>MNRQELITEALKARDMAYAPYSKFQVGAALLTKDGKVYRGCNIENAA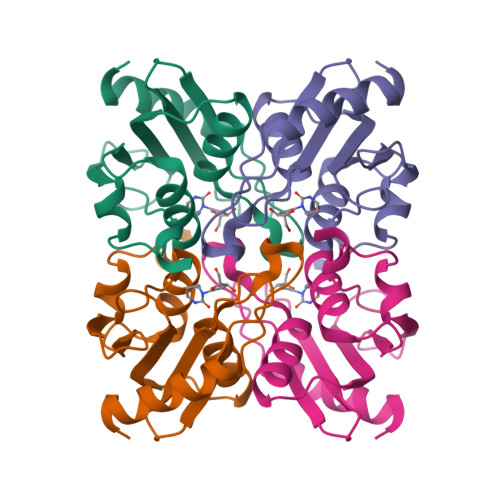YSMCNCAEQTALFKAVSEGDTEFQMLAVAADTPGPVSPCGACRQVISELCTKDVIVVLTNLQGQIKEMTVEELLPGAFSSEDLHDERKL[2x]> DDDDDDDDDDD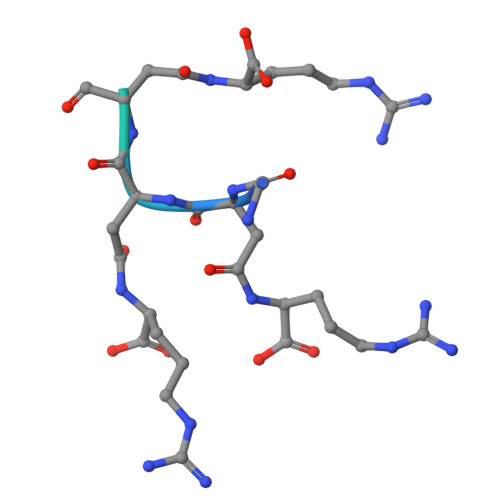DDDDD> NRIITEYILIDANNYHFKSWIECFPDCKVNLKLLLFRPEWFDFFKYVESKTYFPQ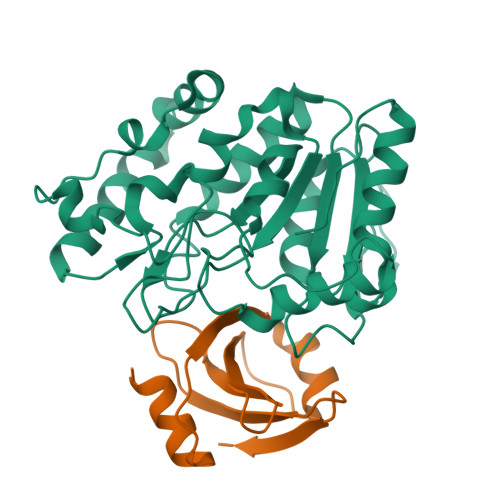LESKLSSYLEKRQRIVPYPELLFNTMNVLPPGKIKVVILGQDPYPGSCISGVPYAMGCSFSVPLNCPVPKSLANIYTNLIKFNHMRKAPKHGCLASWILQGTFMINSAFTTVLNESGVHARTWESFTADLIDYLTDNYDDLIFVAWGAHAHKLCQRVDPKKHYIITSSHPSPLSVSNTMTSMSYGPNPKKVTYPSFNSVDHFGKINEHLKSRNKKPIFWDL;> TNLSDIIEKETGKQLVIQESILMLPEEVEEVIGNKPESDILVHTAYDESTDENVMLLTSDAPEYKPWALVIQDSNGENKIKML>MVRTTKTSMAAASTVAPEVAMDEGSPSTSQAQVELPRNLEVFNEACGHVFGSSFNREDNSVISDAAAFLFKMHTHSLDGQEAKVLRASEKKRERENAKKSRKAPEAGMRVGRSLILTSRWTEYCATCVPALGSKMKVIKASGDAAMIQMMKDHNSLLRVCVRIEVWKARYVSLVALDERIQTLEDAQWFPYLSGDSYRACPGLVGGYFAKKAAAGERGKNYKKLNQTAIIPPPRFLIIGHRLQIGDQVTLRELLASIAWGLCDGVLAECWSPSQGDGSIGVVVGLPLQATGSCFLVVASHGLSAIADS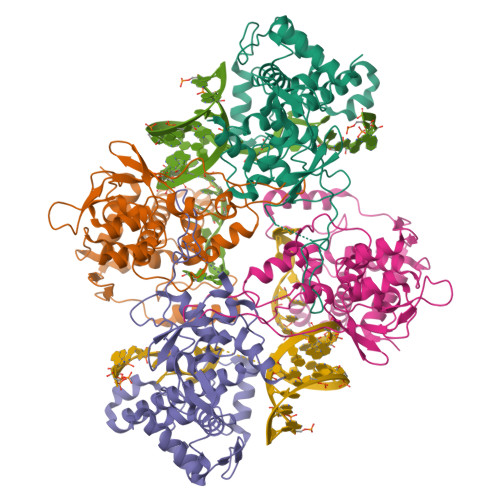RIEGTGNTNLLEECIAIQKQDGVIKCKRSGKSLYHCLKETAGAVGR[4x]> MTKKVGLLVMAYGTPYKDEDIERYYTDIRHGHKPSEEMIADLRGRY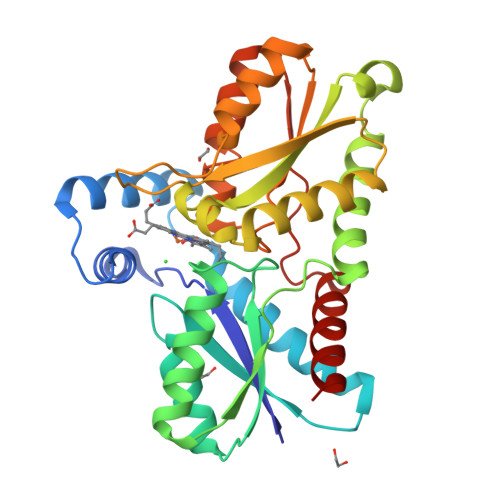HAIGGLSPLAKITEAQAYGLEKALNDSQDEVEFKAYIGLKHIEPFIEDAVEAMHKDGIEEAISIVLAPHYSSFSVEAYNKRAKEAADKLGGPRINAINDWYKQPKFIQMWADRINETAKQIPADELLDTVLIVSAHSLPEKIKQHNDPYPNQLQETADFIFEKVVVPHYALGWQSEGKTGEPWLGPDVQDLTRELYGREKYKHFIYTPVGFVAEHLEVLYDNDYECKVVTDEVGAAYHRPPMPNSDPEFLEVLRTVVWEKYSNLE pmcNeuronal signaling that prompts coughing is well documented and is primarily mediated by ligand-gated ion channels known as P2X3 receptors. These receptors, comprising an extracellular ligand-binding domain and a membrane-spanning ion channel domain, swiftly convert extracellular chemical signals into transmembrane ionic currents, facilitating rapid intercellular signaling and chemosensation. Purinergic P2X3 receptors gated by ATP exist in both homotrimeric (comprising three P2X3 subunits) and heterotrimeric (comprising one P2X2 subunit and two P2X3 subunits, termed P2X2/3) configurations. A single subunit of the P2X3 receptor displayed a distinctive “dolphin-like” shape, akin to the broader P2X receptor family.

Here, we report a cryo-EM structure of camlipixant-bound P2X3, revealing a previously undiscovered selective drug-binding site in the receptor. To resolve the full-length receptor complexed with camlipixant, we employed the peptidisc approach to stabilize the receptor and bind it to camlipixant. Camlipixant binds to the pocket above the ATP-binding site formed by the upper body domain between the adjacent subunits. This drug-binding pocket is encircled by residues that predominantly protrude from the β-strands (β3, β4, β5, β13, and β14). Residues M70, M91, F277, and L293 (subunit A) form a complex network of contacts favoring nonpolar environments, indicating a predominantly hydrophobic binding interface between the receptor and camlipixant. Specifically, R68 (subunit A) and E288 (subunit C) recognize camlipixant by cation–π and charge–charge interactions with the difluorophenyl ring and N04, respectively, acting as a lid in the binding process. Upon camlipixant binding, P2X3 underwent conformational changes, adopting a closed state as indicated by the constriction of the channel gate formed by transmembrane helices at residues I318 and V321. In addition, upon camlipixant binding, the transmembrane helices moved closer to the gate. Camlipixant binding disrupts conformational changes in the upper body domain, including residue Y281, causing insufficient movement of the pore-lining transmembrane helices to simultaneously open the channel. Camlipixant binding induces conformational changes in the extracellular domain machinery that block the ATP-binding site and stabilize the closed ion entry gate.

>[3x]GSDFFTYETTKSVVVKSWTIGVINRAVQLLIISYFVGWVFLHEKAYQVRDTAIESSVVTKVKGFGRYANRVMDVSDYVTPPQGTSVFVIITKMIVTENQMQGFCPESEEKYRCVSDSQCGPQRFPGGGILTGRCVNYSSTLRTCEIQGWCPTEVDTVEMPVMMEAENFTIFIKNSIRFPLFNFEKGNLLPNLTAADMKTCRFHPDKAPFCPILRVGDVVKFAGQDFAKLARTGGVLGIKIGWVCDLDRAWDQCIPKYSFTRLDGVSEKSSVSPGYNFRFAKYYKMENGSEYRTLLKAFGIRFDVLVYGNAGKFNIIPTIISSVAAFTSVGVGTVLCDIILLNFLKGADQYKAKKFEEVDET>GPSKSSSSRRNAW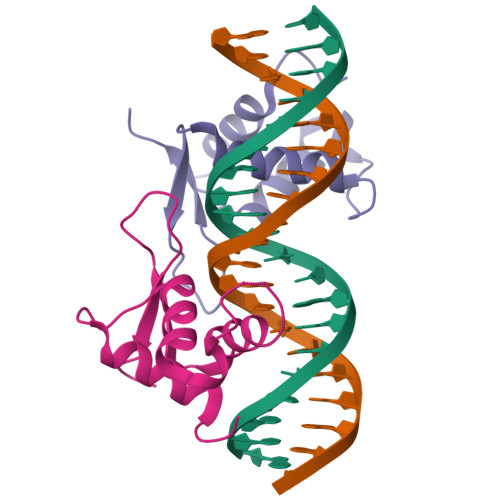GNLSYADLITKAIESSAEKRLTLSQIYEWMVKSVPYFKDKGDSNSSAGWKNSIRHNLSLHSKFIRVQNEGTGKSSWWMLNPEGGKSGKSPRRRAASMDNNSKFAK[6x]> MMKTYKIAVDGPAASGKSSTSDLVARKLGFSHLISGNLYRAVTYGLVRRFGEVRPGDEEQ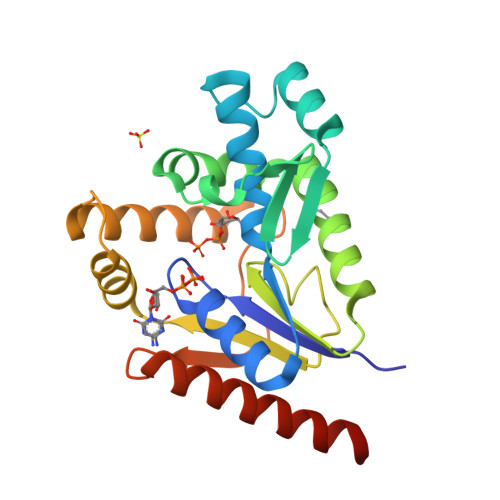KRFVLELSIEVRNNRVFLDGEDVSESLRKEVVDRHVVSVAREKYIREKVFTIQRSVIDLEKRGIVVDGRDIATRIMPNADLKVFLTASPETRARRRYMEGGSESYEELLESIKKRDHNDRTREHDPLVATCDSIVIENDSMTLEETADEIIRLFRRVESFNAGHHHHHH In the Gram-positive pathogenic bacterium Clostridium perfringens the conjugative tetracycline resistance plasmid pCW3 is representative of a large class of closely related toxin and antibiotic resistance plasmids. In this study, we have identified TcpK, a protein encoded by a gene upstream of the oriT site and tcpM, as being a major factor required for the efficient conjugation of the pCW3 plasmid. Our data revealed that TcpK was a distantly related member of the wHTH family of DNA binding proteins. Our data suggest that its function is to decorate the origin of transfer of pCW3 and to interact specifically with sequences that are only present in this region of the plasmid.

To complement these biophysical experiments, we determined the structure of TcpK in complex with the 23 bp region derived from oriT. The asymmetric unit of the crystal contained four TcpK dimers (termed A:B, C:D, E:F, G:H) bound to four 23 bp dsDNA molecules. Superposition of TcpK to its DNA-bound form does not reveal any significant structural changes to the protein (Global r.m.s.d. of 0.40–0.9 Å). However, the DNA molecules have undergone a subtle, but noticeable, twisting induced by TcpK binding. Unexpectedly, each TcpK dimer bridges across two strands of DNA. This result is in contrast to any other known wHTH protein, where the dimer arrangement permits interaction through the canonical helix with palindromic sequences on the same DNA strand. Comparison of the TcpK/DNA complex with these wHTH/DNA assemblies reveals that TcpK interacts with DNA through a novel binding mode. Here the β-wing (β3–β4) sits within the major groove while the canonical helix (H3) only makes a single DNA contact through R60 to the phosphate backbone. Additional residues making contact with the DNA are all located outside the canonical helix. These interactions are through the loops N22-K31 and E69-N73, and, in particular, the sidechain of R28, which stretches into the minor groove. Additionally, the protein makes hydrogen bond interactions with the inter TcpK box bases (-CAG-).

>QNSHMVKDLNLYAKELVDVVNYLMKKNQLVFSRNNKFIYVNTETIKSMLEKRNYDTVDGKLYLWRELEWIECAEDRFNKRIKIDGENMYAVVIKYSSYSILKRLYLE[8x]> MASRYWVVSLPVQNSAASVWNRLQE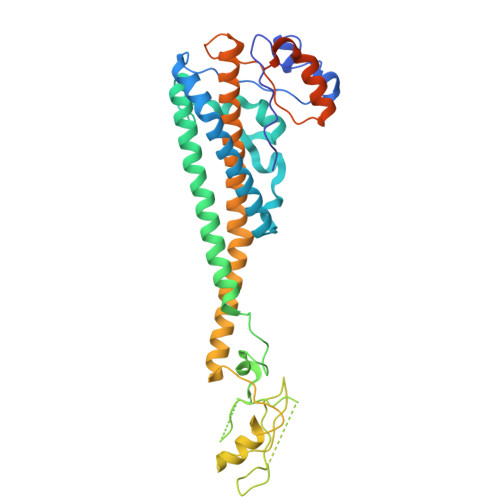QISKHSFDTPLYRFNIPNLRVGTLDSLLALSDDLVKSNSFVESVSHKIRRQIEELERVSGIESSSLSVDGVPVDTYLTRFVWDEAKYPTMSPLREIVDGIHTLVAKIEDDLKVRVAEYNNVRSQLNAINRKQSGSLAVRDLSNLVKPEDIITSEHLVTLLAVVPKYSQKDWLASYETLTSYVVPRSSKLLYEDNEYALYTVTLFGRVADNFRIAAREKGFQIRDFEYSSEAQESRNQELEKLVHDQESLRSSLLQWCYTSYGEVFSSWMHFCAVRVFAESILRYGLPPSFLACVLAPSVKGEKKVRSILEELCGNANSTFWKSEDDGGMMAGLGGDADSHPYVSFTINLV>MGSSHHHHHHSGIDGISSNESNIKIGAAANASHPGGVAAVSVQAAGAPYNAFTGFSSLKGLAQAFAAQGTSNTNVTVGSKTFNISHIPVSAMPPSHSALGNFNFGQVGTQEVYFGEWWKAGDTPASASHTVYYAGDNTNTTVPTAGTATYTVA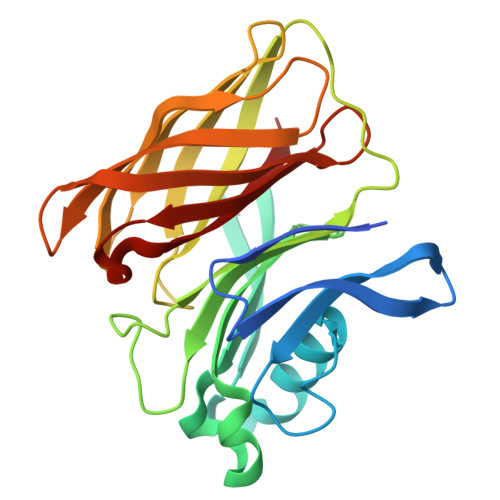GINGSGSNLLSGTFTANYGAGTLEGTLTGTGTAVSSLSLDGVAFNPGTAAFAGLATANGTAGIDNSGVVQGQFFGANASALAGIAQFDNVSYNTAFGGAKN[3x]>[4x]GVKLEERQRIARDLHDTLGQKLSLIG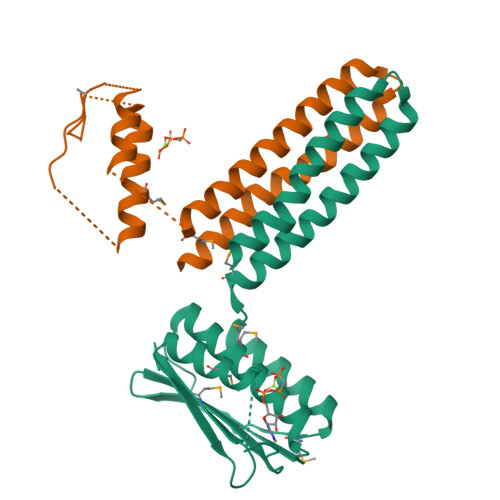LKSDLARKLIYKDPEQAARELKSVQQTARTSLNEVRKIVSSMKGIRLKDELINIKQILEAADIMFIYEEEKWPENISLLNENILSMCLKEAVTNVVKHSQAKTCRVDIQQLWKEVVITVSDDGTFKGEENSFSKGHGLLGMRERLEFANGSLHIDTENGTKLTMAIPNNSK> SEVGKSFKDRKMIEKMQEENRKDREKAAAKFREYFPNFVGEPKSKDILKLRLYEMQHGKCLYSGKEINLGRLNEKGYVEIDHALPFSRTWDDSFNNKVLVLGSENQNKGNQTPYEYFNGKDNSREWQEFKARV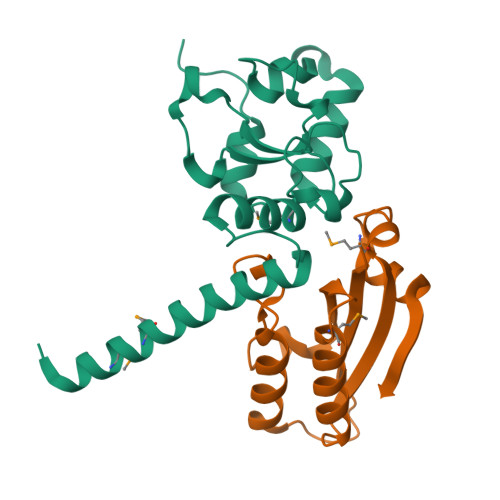ETSRFPRSKKQRILLQKFDEDGFKERNL;> SMAFKRAIIFTSFNGFEKVSRTEKRRLAKIINARVSIIDEYLRAKDTNASLDGQYRAFLFNDESPAMTEFLAKLKAFAESCTGISIDAWEIEESEYVRLPVERRDFLAAANGKEIFKI> MRERTRINVDASEAVRPFNRFWRGTGFSPAELLLEPEMRQMLAYIGGLPNEGIKFLRVHYLYNLLSAKGGAGYDWSLLDRALDVMIEHRLKPFFELMGNPSGLFTDYEDMDQVRRWRDLVTATVDRYGARYGMDELRTWYFETTNQADSGWWTYGIKGYTNYYDACVAGLDAIDPSLPMGGPGTARTLSPIFRALMAHCDSGTSCLTGDGPPRIDYISIHEKGV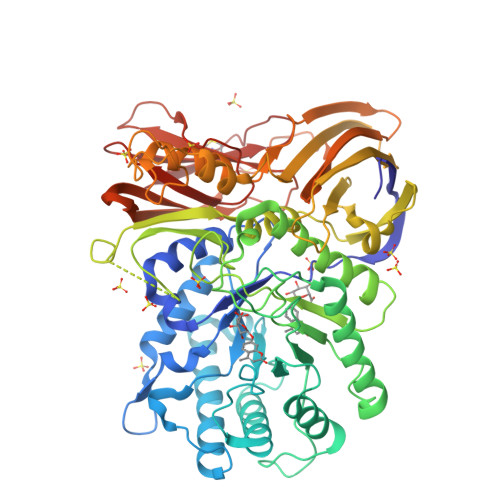NGSKEDLTPKTNAIVDRTLLVVDYLKEHHPRLAGLPIVNDECDPQLGWSDHHSWHGKAYYAGIIARIIEQHDRRIIAPKAANFTFLSSDHAFIGGWSQRTIFAYFGSRNFTKAQWEHKTNLDMLVTDVDRTPPFDIIKKPGLTSMELLATLGDTVCKVTAEPPLDPDQDGLAILPTRLPGGGVSISLIHSVDAINRSGRTAVRLEVSGLVPGRHAICLLRIDEEFTNPMEVWEAQRDESNPRGPFEPVGAPPAPTEAQFAELRRAQEPALLHPISVVACDEGRISVDLDVPLPSLTQVLVVPDVGVPPAAPTGLVVERYLGLGGREERMLFWAAGDISPAIFYDVLVSTDGGTFEKVSSAPLISTAFLHMSPPEGVRYAVCARDAFGRRSELCLSRS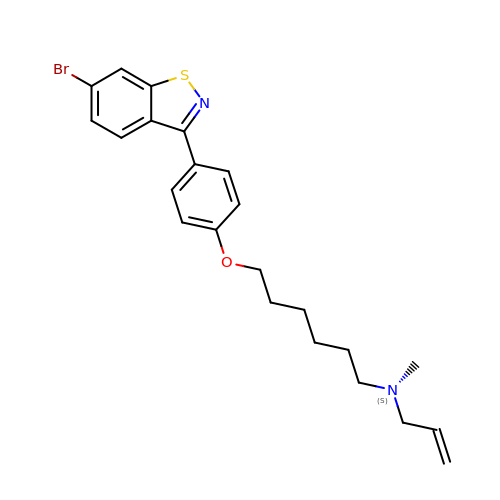N-{6-[4-(6-BROMO-1,2-BENZISOTHIAZOL-3-YL)PHENOXY]HEXYL}-N-METHYL-2-PROPEN-1-AMINE | C23 H27 Br N2 O S | ZHDHSBKTLRLUCQ-UHFFFAOYSA-N>[4x]MVANPEHYIKHPLQNRWALWFFKNDKSKTWQANLRLISKFDTVEDFWALYNHIQLSSNLMPGCDYSLFKDGIEPMWEDEKNKRGGRWLITLNKQQRRSDLDRFWLETLLCLIGESFDDYSDDVCGAVVNVRAKGDKIAIWTTECENRDAVTHIGRVYKERLGLPPKIVIGYQSHADTATKSGSTTKNRFVV

In addition, the cap fulfills numerous other biological functions that are mediated by specific cap-binding proteins and include maturation, transport, and eIF4E-mediated translation initiation. Upon binding the cap, the eIF4E protein changed its conformation from open to closed, bringing the Trp102 and Trp56 closer to the cap, and together with the structural water molecules, stapling the ligand with the protein structure. Finally, to gain more insight into the consequences at the molecular level of N7-benzylation of the mRNA cap, we determined the crystal structures of three compounds with eIF4E. Overall, the comparison of these three crystal structures indicated that different benzyl substituents can be accommodated in the cap binding pocket due to (i) the conformational flexibility of Trp102, which was also previously observed for m7GMP analogs, and (ii) the presence of structural water molecules in the N7-methyl-binding cavity, which could be replaced upon introduction of larger hydrophobic substituents.

Crystal structures were refined using diffraction data to the resolution of 2.2 Å for 1a, 2.67 Å for 1c, and 2.66 Å for 1h. In contrast, in the complex with the 3-methylbenzyl dinucleotide (1c), Trp102 was pushed out from the binding pocket, disrupting the stacking interaction, which was most likely the cause of decreased binding affinity for this compound. In the case of the benzyl modified cap 1a, for which the benzyl ring was directed upwards, most of the structural water molecules were conserved in the cavity, while for 3-MeBn7GpppG and 4-Cl-Bn7GpppG the benzyl rings were directed downwards into the cavity, and the structural water molecules were replaced by 3-methylbenzyl rings or 4-chlorobenzyl substituents. The guanosine of 4-Cl-Bn7GpppG was not visible in the crystal structure, while the guanosines of Bn7GpppG and 3-MeBn7GpppG were stabilized by interactions with amino acids from the loop comprised of residues 50–59. Specifically, backbone carbonyl oxygen atoms of lysine 54 and 52 formed hydrogen bonds with N1 and N2 of guanine, respectively, and amide group (NH2) of Asn59 was a donor in a hydrogen bond with O6 of guanosine. For the eIF4E complex with 4-Cl-Bn7GpppG (1h), in which 4-chlorobenzyl appeared to be stabilized via polar contacts in the cavity, the phosphate chain could adopt two conformations, wherein one imitated the phosphate chain of m7GpppG, while in the Bn7GpppG (1a) and 3-MeBn7GpppG (1c) complexes, γ and β phosphates were shifted out of the pocket by 2–3 Å (distances measured between corresponding phosphorus atoms). Consequently, this weakened the interaction of the phosphate chain with the positively charged side chains of Arg157 and Lys162, mitigating the potential stabilization introduced by additional hydrophobic interactions of the benzyl group.> GPLGSMDDGSVSDIKRGRAARNAKLASIPVGFAGRAALGLGKRLTGKSKDEVTAELMEKAANQLFTVLGELKGGAMKVGQALSVMEAAIPDEFGEPYRE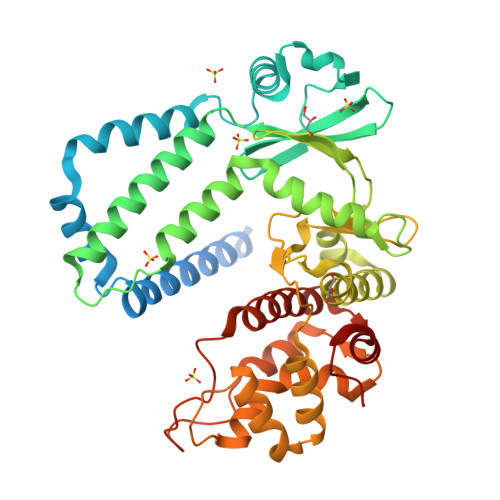ALTKLQKDAPPLPASKVHRVLDGQLGTKWRERFSSFNDTPVASASIGQVHKAIWSDGREVAVKIQYPGADEALRADLKTMQRMVGVLKQLSPGADVQGVVDELVERTEMELDYRLEAANQRAFAKAYHDHPRFQVPHVVASAPKVVIQEWIEGVPMAEIIRHGTTEQRDLIGTLLAELTFDAPRRLGLMHGDAHPGNFMLLPDGRMGIIDFGAVAPMPGGFPIELGMTIRLAREKNYDLLLPTMEKAGLIQRGRQVSVREIDEMLRQYVEPIQVEVFHYTRKWLQKMTVSQIDRSVAQIRTARQMDLPAKLAIPMRVIASVGAILCQLDAHVPIKALSEELIPGFAEPDAIVV>HHHHHHVEDATRSDSTTQMSSTPEVVYSSAVDSKQNRTSDFDANWKFMLSDSVQAQDPAFDDSAWQQVDLPHDYSITQKYSQSNEAESAYLPGGTGWYRKSFTIDRDLAGKRIAINFDGVYMNATVWFNGVKLGTHPYGYSPFSFDLTGNAKFGGENTIVVKVENRLPSSRWYSGSGIYRDVTLTVTDGVHVGNNGVAIKTPSLATQNGGNVTMNLTTKVANDTEAAANITLKQTVFPKGGKTDAAIGTVTTASKSIAAGASADVTSTITAASPKLWSIKNPNLYTVRTEVLNGDTVLDTYDTEYGFRWTGFDATSGFSLNGEKVKLKGVSMHHDQGSLGAVANRRAIERQVEILQKMGVNSIRTTHNPAAKALIDVCNEKGVLVVEEVFDMWNRSKNGNTEDYGKWFGQTIAGDNAVLGGDKDETWAKFDLTSTINRDRNAPSVIMWSLGNEMMEGISGSVSDFPATSAKLVAWTKAADSTRPMTYGDNKIKANWNESNTMGDNLTANGGVVGTNYSDGANYDKIRTTHPSWAIYGSETASAINSRGIYNRTTGGAQSSDKQLTSYDNSAVGWGAVASSAWYDVVQRDFVAGTYVWTGFDYLGEPTPWNGTGSGAVGSWPSPKNSYFGIVDTAGFPKDTYYFYQSQWNDDVHTLHILPAW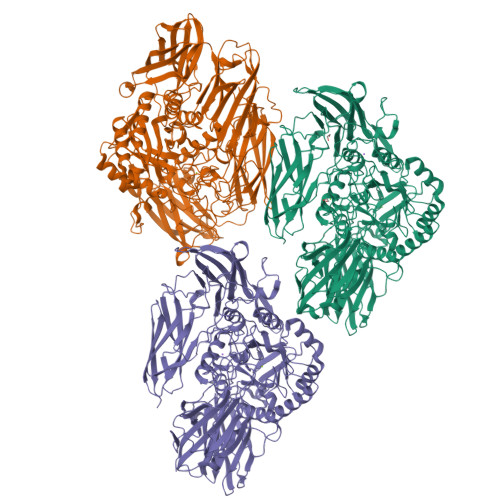NENVVAKGSGNKVPVVVYTDAAKVKLYFTPKGSTEKRLIGEKSFTKKTTAAGYTYQVYEGTDKDSTAHKNMYLTWNVPWAEGTISAEAYDENNRLIPEGSTEGNASVTTTGKAAKLKADADRKTITADGKDLSYIEVDVTDANGHIVPDAANRVTFDVKGAGKLVGVDNGSSPDHDSYQADNRKAFSGKVLAIVQSTKEAGEITVTAKADGLQSSTVKIATTAVPGTSTEKTVRSFYYSRNYY[3x]> MRNEMHLQFSARSENESFARVTVAAFVAQLDPTMDELTEIKTVVSEAVTNAIIHGYNNDPNGIVSISVIIEDGVVHLTVRDEGVGIPDIEEARQPLFTTKPELERSGMGFTIMENFMDEVIVESEVNKGTTVYLKKHGIHHHHHH;> MSLAIDLEVKQDVLIVRLSGELDHHTAEELRE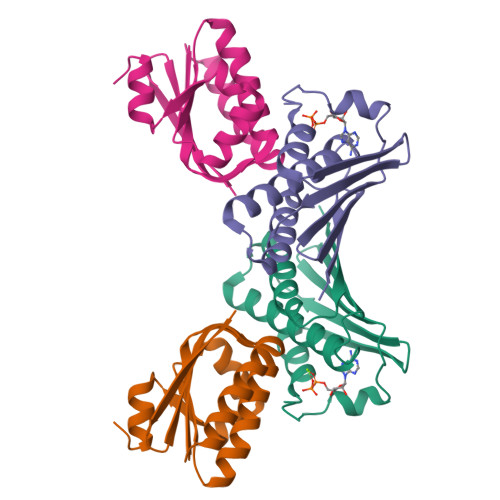QVTDVLENRAIRHIVLNLGQLTFMDSSGLGVILGRYKQIKNVGGQMVVCAVSPAVKRLFDMSGLFKIIRVEADEQFALQALGVA>[6x]MLLSDRDLRAEISSGRLGIDPFDDTLVQPSSIDVRLDCLFRVFNNTRYTHIDPA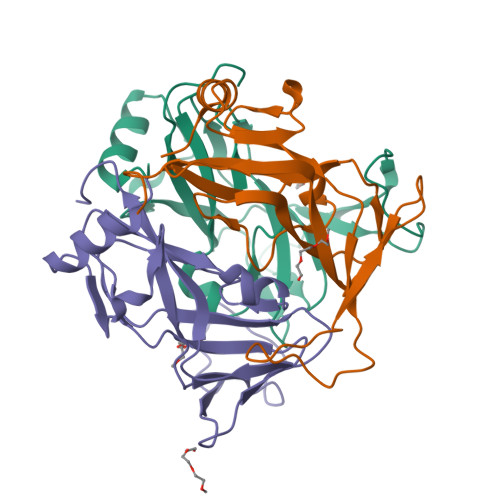KQQDELTSLVQPVDGEPFVLHPGEFVLGSTLELFTLPDNLAGRLEGKSSLGRLGLLTHSTAGFIDPGFSGHITLELSNVANLPITLWPGMKIGQLCMLRLTSPSEHP> PTHADSLNNLANIKREQGNIEEAVRLYRKALEVFPEFAAAHSNLASVLQQQGKLQEALMHYKEAIRISPTFADAYSNMGNTLKEMQDVQGALQCYTRAIQINPAFADAHSNLASIHKDSGNIPEAIASYRTALKLKPDFPDAYCNLAHCLQIVCDWTDYDERMKKLVSIVADQLEKNRLPSVHPHHSMLYPLSHGFRKAIAERHGNLCLDKINVLHKPPYEHPKDLKLSDGRLRVGYVSSDFGNHPTSHLMQSIPGMHNPDKFEVFCYALSPDDGTNFRVKVMAEANHFI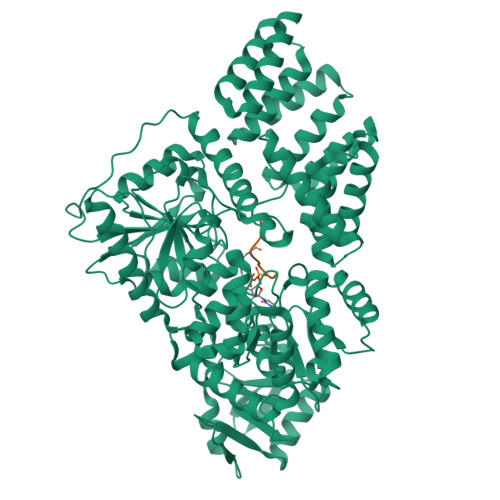DLSQIPCNGKAADRIHQDGIHILVNMNGYTKGARNELFALRPAPIQAMWLGYPGTSGALFMDYIITDQETSPAEVAEQYSEKLAYMPHTFFIGDHANMFPHLKKKAVIDFKSNGHIYDNRIVLNGIDLKAFLDSLPDVKIVKMKCPDGGDNADSSNTALNMPVIPMNTIAEAVIEMINRGQIQITINGFSISNGLATTQINNKAATGEEVPRTIIVTTRSQYGLPEDAIVYCNFNQLYKIDPSTLQMWANILKRVPNSVLWLLRFPAVGEPNIQQYAQNMGLPQNRIIFSPVAPKEEHVRRGQLADVCLDTPLCNGHTTGMDVLWAGTPMVTMPGETLASRVAASQLTCLGCLELIAKNRQEYEDIAVKLGTDLEYLKKVRGKVWKQRISSPLFNTKQYTMELERLYLQMWEHYAAGNKPDHMIKPVE> MGHHHHHHGGMSNWTTYPQKNLTQAEQLAQLIKEADALVVGIGAGMSAADGFTYIGPRFETAFPDFIAKYQFLDMLQASLFDFEDWQEYWAFQSRFVALNYLDQPVGQSYLDLKEILETKDYHIITTNADNAFWVAGYDPHNIFHIQGEYGLWQCSQHCHQQTYKDDTVIRQMIAEQKNMKVPGQLIPHCPECEAPFEINKRNEEKGMVEDADFHAQKARYEAFLSEHKEGKVLYLEIGVGHTTPQFIKHPFWKRVSENPNALFVTLNHKHYRIPLSIRRQSLELTEHIAQLISATKTIYQKS

In this study, we report on the identification of a distinct class of sirtuins (SirTMs) found primarily in pathogenic microorganisms and show that these function as protein ADP-ribosyl transferases. Members of this sirtuin class are genetically linked to a specific subclass of macrodomain proteins, which reverse the sirtuin catalyzed ADP-ribosylation. Moreover, we show that in Staphylococcus aureus and Streptococcus pyogenes the sirtuin-mediated ADP-ribosylation is dependent on another posttranslational modification—lipoylation.

To gain further insight into the SirTM catalyzed ADP-ribosylation, we determined the crystal structure of SpySirTM, both in the ligand-free form as well as bound to ADPr or NAD+. The overall fold for these three structures is identical with a low root-mean-square deviation (RMSD) (0.29–0.31 Å). The models contain residues 3–292 (residues 7–10 are not visible in the electron density maps) and follow a typical sirtuin fold comprised of a large Rossmann fold and a small bipartite zinc coordinating domain. No major conformational changes are observed upon binding of either ADPr or NAD+, with the exception of slight readjustment of the loop region between β6 and α14 as well as following β7. The most surprising difference is the replacement of the absolutely conserved HG motif containing the catalytic H residue by QG. In accordance with the functional analysis, our sequence and structural analysis revealed the absence of a catalytic histidine residue, crucial for the proposed deacylase mechanism and found in all other hitherto described sirtuins and that may explain the apparent absence of deacylation activity in SirTMs.>MASWSHPQFEKMGMLEARELLCERDERTLFSGLSFTLNAGEWVQITGSNGAGKTTLLRLLTGLSRPDAGEVLWQGQPLHQVRDSYHQNLLWIGHQPGIKTRLTALENLHFYHRDGDTAQCLEALAQAGLAGFEDIPVNQLSAGQQRRVALARLWLTRATLWILDQPFTAIDVNGVDRLTQRMAQHTEQGGIVILTTHQPLNVAESKIRRISLTQTRAA[2x];>[2x]MMFWRIFRLELRVAFRHSAEIANPLWFFLIVITLFPLSIGPEPQLLARIAPGIIWVAALLSSLLALERLFRDDLQDGSLEQLMLLPLPLPAVVLAKVMAHWMVTGLPLLILSPLVAMLLGMDVYGWQVMALTLLLGTPTLGFLGAPGVALTVGLKRGGVLLSILVLPLTIPLLIFATAAMDAASMHLPVDGYLAILGALLAGTATLSPFATAAALRISIQ;> MWKTLHQLAIPPRLYQICGWFIPWLAIASVVVLTVGWIWGFGFAPADYQQGNSYRIIYLHVPAAIWSMGIYASMAVAAFIGLVWQMKMANLAVAAMAPIGAVFTFIALVTGSAWGKPMWGTWWVWDARLTSELVLLFLYVGVIALWHAFDDRRLAGRAAGILVLIGVVNLPIIHYSVEWWNTLHQGSTRMQQSIDPAMRSPLRWSIFGFLLLSATLTLMRMRNLILLMEKRRPWVSELILKRGRK;> MTPAFASWNEFFAMGGYAFFVWLAVVMTVIPLVVLVVHSVMQHRAILRGVAQQRAREARLRAAQQQEAA

Here we report cryo-electron microscopic structures of the heme translocation complex CcmABCD from E. coli, alone and bound to the heme chaperone CcmE. CcmABCD forms a heterooctameric complex centered around the ABC transporter CcmAB that does not by itself transport heme. Our data suggest that the complex flops a heme group from the inner to the outer leaflet at its CcmBC interfaces, driven by ATP hydrolysis at CcmA. A conserved heme-handling motif (WxWD) at the periplasmic side of CcmC rotates the heme by 90° for covalent attachment to the heme chaperone CcmE that we find interacting exclusively with the CcmB subunit.

No heme was bound in this sample, and we obtained one data set that contained CcmA without and one with bound ATP, with only minor changes to the overall conformation of the complex. The binding sites for ATP were located close to the interface of the CcmA dimer, with residue S130 from the other monomer involved in the coordination of the ATP phosphates. ATP bound to its canonical position in this class of proteins, with the P-loop cradling the triphosphate near the switch I and switch II regions and the lid loop. The overall conformational changes in the different states of CcmA were subtle, and the nucleotide-free wild-type structure showed the same conformation of the P-loop as the nucleotide-free E154QA variant, although the latter switched the transporter into its closed state. Only upon binding of MgATP the conformation of the P-loop changed substantially, including in the lid loop where H83 coordinated the Mg2+ cation. Unexpectedly, the overall stoichiometry of the CcmABCD changed for the E154QA variant, in that the closure of the core ABC transporter Ccm(AB)2 consistently led to the loss of one copy of CcmCD, resulting in a Ccm(E154QAB)2CD complex. In contrast, the observed conformational change of the outer protomer of CcmB in the ATP-bound state or the E154QA variant complex implies that an adjacent CcmC protomer would have to either dissociate from the complex or change its own conformation in response. The closure of the dimeric transporter induced a conformational change of helices hI and hV in only one monomer of the CcmB dimer that is not compatible with the observed binding mode of CcmC to CcmB, as on the cytoplasmic side of the membrane, helix hV of CcmB was pushed outward, leading to a clash with helix hIV of CcmC. It seems feasible that such a rearrangement results in the effective ejection of the CcmCD module from the complex, and it is quite remarkable that it occurs only in one protomer of the CcmB dimer, while the other almost completely retains its open-state conformation with CcmCD in place. The model had the core ABC transporter Ccm(AB)2 in a closed state, very similar to the ATP-bound E154QA variant complex.>MVKVDLESKRYGEKLKEVFLMLDNNVVECIKEITESSRNGKLVFFVGAGVSTLSDYPQWWRLVDKYHEELYGSPKKGNYSSDEYLRIPQIFYNVKGEMAFDGILKDFFQVDKPTNPIHDKILAMNPAHVITTNYDNLIDTACWKRGKYFSVISAEEDVANATSSRYLLKVAGDFRKGFKGENVVLKEDDYLNYDQNYPLISNLMKTIIATHTIVFIGYGLGDYNINMLLNWVRKLQKDSFHKPFFIRTDPSPIENETLIYYENKGLRIIDAASLIDSNEYDYLERYSAVMDLLIESQENKFITKDDEVIDYIYGKISPLFALQYIRKIDLKHVFEYDYHFEVNGTVVRHKNKGFGYMERFFELKESCDERSKLSKKQYERFNALFNFFEKNGVICMAKDAGTLNTSIEINSLAYHGKYDVMKKFIEEQSVSIEDDYKKAFFLACLGRWEESYDLYSNIILNSIDESNGCVYYLSQINRYRIYQSITQAVTQFNGLGLLTFGRHYKPFTDEFLARIEREMTNFNIDDLFNGMPFEFQKKYKILEFLSDNQFLYDDTVKLFELTNKVRSEMSEGSYSFGMSSDIVVLLRLYDNLRFLYENCLWSVSFHEFHQYIRNSMSLLIEKAEYERTRDIDELGFSFFGKKSGFFMEYYDFVNISRHFKIDDIKNLERSCSIDKIRFGEQEKIEEYLVGIAEEITKQFSANGMNVVFYTQFISEAKAALYFAKYVKLSEEGLGKIVKALLFYFPERDLDIGKRYVWLERLTKCNELPKSIISIIDDFLVLQAEKHIDQNYSEVSSNGLYSRDYGALIKHFEKNFISKRLSEITLCLTQDKQKQIDFLFKLLPLLSTNAKSHLLSFKSVENINDLMNGIRIGLIDEFTPEHEELIIEYLETRKVNYIVEKEKGIQTFSSNDYMSTFGIWYFLEEINNSKMEEFIGMDDQYDFFVDPENFDYKKFIPSWLKNYNDKLLGKIAGNKHMKHHVIEVLKERVKNSNDK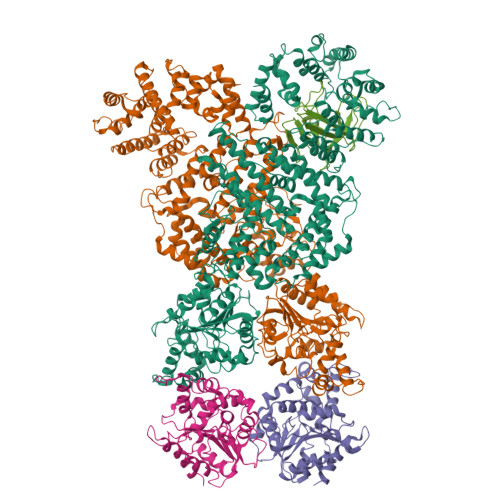RYLEILMNYFI[4x];> KDTGATHDLVYHSKINTFVWDVEFDIVLSDSKELNKCYFVKCFNPYRINGKCDFAVSSIDIFSEGKRLLIENEFNFKITKAVHVATSKDVTEIVLHLSERISSPFPIVKEVVYLD>MCGIFAYLNYHVPRTRREILETLIKGLQRLEYRGYDSAGVGFDGGNDKDWEANACKIQLIKKKGKVKALDEEVHKQQDMDLDIEFDVHLGIAHTRWATHGEPSPVNSHPQRSDKNNEFIVIHNGIITNYKDLKKFLESKGYDFESETDTETIAKLVKYMYDNRESQDTSFTTLVERVIQQLEGAFALVFKSVHFPGQAVGTRRGSPLLIGVRSEHKLSTDHIPILYRTGKDKKGSCNLSRVDSTTCLFPVE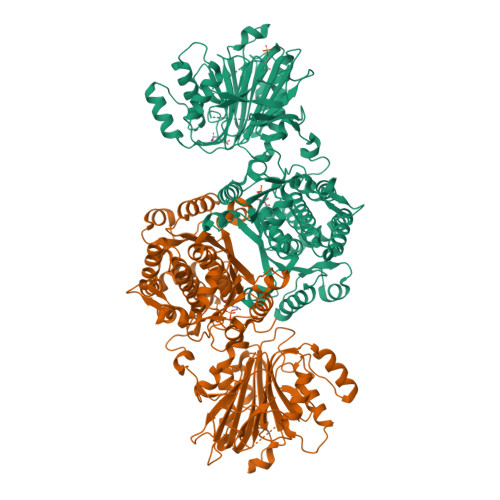EKAVEYYFASDASAVIEHTNRVIFLEDDDVAAVVDGRLSIHRIKRTAGHHHHHHDHPGRAVQTLQMELQQIMKGNFSSFMQKEIFEQPESVVNTMRGRVNFDDYTVNLGGLKDHIKEIQRCRRLILIACGTSYHAGVATRQVLEELTELPVMVELASDFRDRNTPVFRDDVCFFLSQSGETADTLMGLRYCKERGALTVGITNTVGSSISRETDCGVHINAGPEIGVASTKAYTSQFVSLVMFALMMCDDRISMQERRKEIMLGLKRLPDLIKEVLSMDDEIQKLATELYHQKSVLIMGRGYHYATCLEGALKIKEITYMHSEGILAGELKHGPLALVDKLMPVIMIIMRDHTYAKCQNALQQVVARQGRPVVICDKEDTETIKNTKRTIKVPHSVDCLQGILSVIPLQLLAFHLAVLRGYDVDFPRNLAKSVTVE[2x]>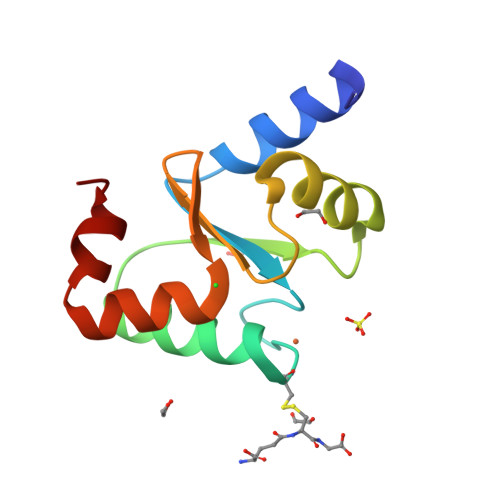[2x]SMAPKLEERLKVLTNKASVMLFMKGNKQEAKCGFSKQILEILNSTGVEYETFDILEDEEVRQGLKAYSNWPTYPQLYVKGELVGGLDIVKELKENGELLPILRGE The ciliary protein Arl3 has been shown to act as a specific release factor for myristoylated and farnesylated ciliary cargo molecules by binding to the effectors Unc119 and PDE6δ. Here we describe a newly identified Arl3 binding partner, CCDC104/CFAP36. Biochemical and structural analyses reveal that the protein contains a BART-like domain and is called BARTL1. It recognizes an LLxILxxL motif at the N-terminal amphipathic helix of Arl3, which is crucial for the interaction with the BART-like domain but also for the ciliary localization of Arl3 itself.

Here, we demonstrate by X-ray structure determination that BARTL1 binds Arl3∙GppNHp in a similar fashion to BART complexing Arl2∙GTP (Zhang et al., 2009). The asymmetric unit contained two Arl3∙GppNHp and two BARTL1133 molecules. BARTL1133 displays the same all-helical fold as seen in BART (Zhang et al., 2009). In addition, BARTL1 completely buries the N-terminal helix of Arl3 (area 1). The hydrophobic side of the N-terminal amphipathic helix of Arl3 is buried in a hydrophobic groove formed by helices α3, α4, α4′, and α5 of BARTL1. Alignment of the Arl3 N-terminal sequence of different species shows a conserved LLxILxxL motif. The second interface area is formed by switch I, switch II, and residues of the interswitch toggle of Arl3, and on the BARTL1133 side by the loop connecting α2 and α3 as well as parts of the α3 and α6 helices (area 2). Hydrophobic interactions involving Phe51A and Ile53A of β2, Trp66A of β3, Ile74A, Tyr81A in switch II, and Phe106B of α6, and Leu48B and Thr51B of α3 seem to be important. Since the mutant protein Arl3F51A shows a similar drastic, more than 100-fold loss of affinity, we can conclude that both contact areas make significant contributions to the affinity of the interaction. Therefore, both BART and BARTL1 form a group of Arl2/3 effectors displaying an all-helical BART domain with an unconventional recognition mode involving the binding of the N-terminal helix of Arl2/3 apart from the switches.

>[2x]MGLLSILRKLKSAPDQEVRILLLGLDNAGKTTLLKQLASEDISHITPTQGFNIKSVQSQGFKLNVWDIGGQRKIRPYWRSYFENTDILIYVIDSADRKRFEETGQELTELLEEEKLSCVPVLIFANKQDLLTAAPASEIAEGLNLHTIRDRVWQIQSCSALTGEGVQDGMNWVCKNVNAKKKLEHHHHHH;> GPMAAEEEDEVEWVVESIAGFLRGPDWSIPILDFVEQKCEVFDDEEESKLTYTEIHQEYKELVEKLLESYLKEIGINEDQFQEACTSPLAKTRTSQAILQPVLAAEDFTIFKAMMVQKNIEMQLQAIRIIQERNG;> MAAEEEDEVEWVVESIAGFLRGPDWSIPILDFVEQKCEVFDDEEESKLTYTEIHQEYKELVEKLLESYLKEIGINEDQFQEACTSPLAKTRTSQAILQPVLAAEDFTIFKAMMVQKNIEMQLQAIRIIQERNG> SNFE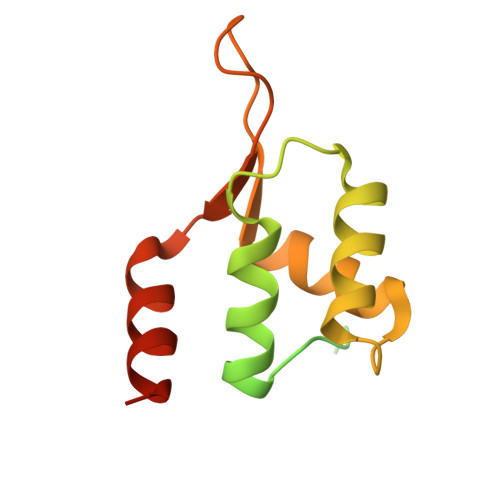NLSEENKRYLQQLKAEVIIETDGPIDPFKEPKTSSLPSKRSNSDLQAQTASQSQSPEKKQKAMITDPMDLLRLFDGVQDSTFSLGTVTEIAQKNLPQYNKQTIKNTIKEYAIRSSGKGDLPRKWVIKDAQNWENLRANANMPTPSL> MAHHHHHHMNILQEPIDFLKKEELKNIDLSQMSKKERYKIWKRIPKCELHCHLDLCFSADFFVSC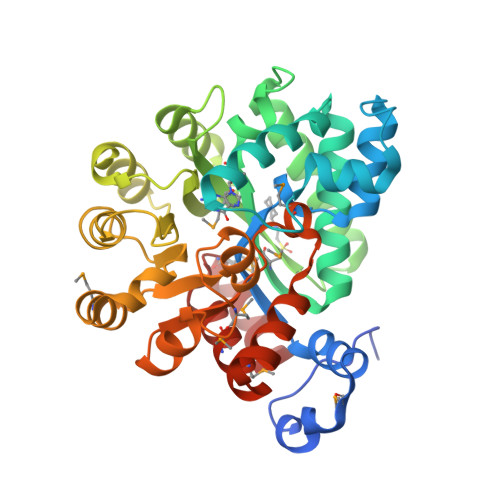IRKYNLQPNLSDEEVLDYYLFAKGGKSLGEFVEKAIKVADIFHDYEVIEDLAKHAVFNKYKEGVVLMEFRYSPTFVAFKYNLDIELIHQAIVKGIKEVVELLDHKIHVALMCIGDTGHEAANIKASADFCLKHKADFVGFDHGGHEVDLKEYKEIFDYVRESGVPLSVHAGEDVTLPNLNTLYSAIQVLKVERIGHGIRVAESQELIDMVKEKNILLEVCPISNVLLKNAKSMDTHPIRQLYDAGVKVSVNSDDPGMFLTNINDDYEELYTHLNFTLEDFMKMNEWALEKSFMDSNIKDKIKNLYF> GPMVKPIPAEGIKSNPSKRHRDRLNTELDRLASLLPFPQDVINKLDKLSVLRLSVSYLRAKSF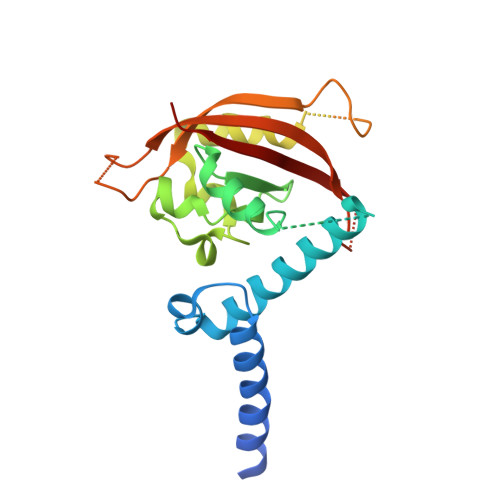FDVALKSSPTERNGGQDNCRAANFREGLNLQEGEFLLQALNGFVLVVTTDALVFYASSTIQDYLGFQQSDVIHQSVYELIHTEDRAEFQRQLHWALNPSQCTESGQGIEEATGLPQTVVCYNPDQIPPENSPLMERCFICRLRCLLDNSSGFLAMNFQGKLKYLHGQKKKGKDGSILPPQLALFAIATPLQ>[2x]MFEQRVNSDVLT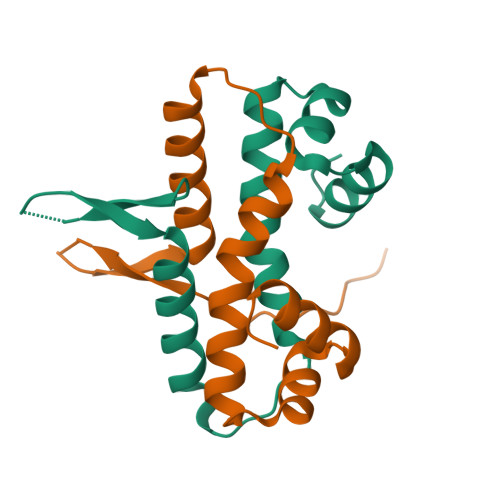VSTVNSQDQVTQKPLRDSVKQALKNYFAQLNGQDVNDLYELVLAEVEQPLLDMVMQYTLGNQTRAALMMGINRGTLRKKLKKYGMN A glucosylglycerate hydrolase (GgH) identified in M. hassiacum and found to be highly conserved among rapidly growing mycobacteria is likely to be responsible for the rapid mobilization of GG accumulated during nitrogen starvation by hydrolysing it to glucose and glycerate. The MhGgH monomer displays an (α/α)6-barrel domain typical of glycoside hydrolase family 63 (GH63), to which MhGgH belongs. While the active site of GH63 members acting on larger substrates is located in an open, solvent-accessible cleft, those of MhGgH and of MgH from T. thermophilus are covered by a cap domain (subdivided into A′- and B′-regions) with constrained access through a narrow negatively charged tunnel. The crystallographic structure of MhGgH revealed a homotetrameric architecture, which is compatible with the oligomeric organization of the enzyme in solution as assessed by SAXS.

To avoid substrate hydrolysis during crystallization or soaking, three catalytically inactive variants of MhGgH were produced. The sequence variations were identified by homology to other characterized MgH enzymes and analysis of the MhGgH–Ser–GOL ternary-complex structure. Two putative catalytic residues (Asp182 and Glu419) and one substrate-interacting residue (Asp43) were identified and replaced by alanine to produce the D43A, D182A and E419A variants. The thermal stability of the D182A and E419A variants was comparable to that of wild-type MhGgH, while that of the D43A variant was slightly lowered (3°C) [Fig. 2(d)].

>GAMPHDPSFTPTQLAARAAYLLRGNDLGTMTTAAPLLYPHMWSWDAAFVAIGLAPLSVERAVVELDTLLSAQWRNGMIPHIVFANGVDGYFPGPARWATATLADNAPRNRLTSGITQPPVHAIAVQRILEHARTRGRSTRAVAEAFLDRRWGDLMRWHRWLAECRDRNERGRITLYHGWESGMANSPRWDSAYANVVPGKLPEYQRADNVIITDPSQRPSDGEYDRYLWLLEEMKAVRYDDERLPSVMSFQVEDVFFSAIFSVACQVLAEIGEDYKRPHADVKDLYLWAERFRAGVVETTDQRTGAARDFDVLAEKWLVTETAAQFAPLLCGGLPHDRERALLKLLEGPRFCGHPDLKYGLIPSTSPVSRDFRPREYWRGPVWPVLTWLFSWCFARRGWAERARLLRQEGLRQASDGSFAEYYEPFTGEPLGSMQQSWTAAAVLDWLG[2x]>[3x]MSDIFNSPQNKASILTALMKSTTGDVEDVLIPKRFRPAKDPLDSPQAAAQFLKDNKYRILRPRAIPTMVELETDAALPRLRQMVEDGKLKDTVSVPEGTTAFYPKYYPFHKPDHDEVGTFGAPDITLLKQLTFFLLENDFPTGPETLRQVREAIATLQYGSGSYSGQLNRLLAMKGVATGRNPNKTPKTVGYTNEQLAKLLEQTLPINTPKHEDPDLRWAPSWLINYTGDLSTDKSYLPHVTIKSSAGLPYIGKTKGDTTAEALVLADSFIRDLGRAATSADPEAGVKKTITDFWYLSCGLLFPKGERYTQVDWDKKTRNIWSAPYPTHLLLSMVSTPVMNESKLNITNTQTPSLYGFSPFHGGMDRIMTIIRDSLDNDEDLVMIYADNIYILQDNTWYSIDLEKGEANCTPQHMQAMMYYLLTRGWTNEDGSPRYNPTWATFAMNVAPSMVVDSSCLLMNLQLKTYGQGSGNAFTFLNNHLMSTIVVAEWVKAGKPNPMTKEFMDLEEKTGINFKIERELKNLRETIVEAVETAPQDGYLADGSDLPPIRPGKAVELDLLGWSAIYSRQMEMFVPVLENERLIASAAYPKGLENKALARKPGAEIAYQIVRYEAIRLVGGWNNPLLETAAKHMSLDKRKRLEVKGIDVTGFLDDWNNMSEFGGDLEGITLSEPLTNQTLVDINTPLDSFDPKARPQTPRSPKKTLDE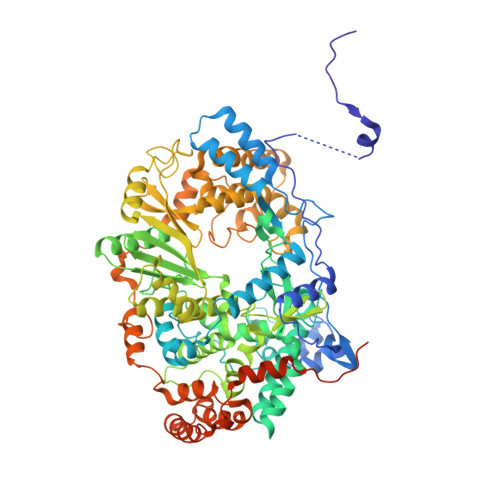VTTAITSGTYKDPKSAVWRLLDQRTKLRVSTLRDQALALKPASSSVDNWAEATEELAQQQQLLMKANNLLKSSLTETREALETIQSDKIIAGKSNPEKNPGTAANPVVGYGEFSEKIPLTPTQKKNAKRREKQRRNQVEHHHHHH;> MSDIFNSPQNKASILTALMKSTTGDVEDVLIPKRFRPAKDPLDSPQAAAQFLKDNKYRILRPRAIPTMVELETDAALPRLRQMVEDGKLKDTVSVPEGTTAFYPKYYPFHKPDHDEVGTFGAPDITLLKQLTFFLLENDFPTGPETLRQVREAIATLQYGSGSYSGQLNRLLAMKGVATGRNPNKTPKTVGYTNEQLAKLLEQTLPINTPKHEDPDLRWAPSWLINYTGDLSTDKSYLPHVTIKSSAGLPYIGKTKGDTTAEALVLADSFIRDLGRAATSADPEAGVKKTITDFWYLSCGLLFPKGERYTQVDWDKKTRNIWSAPYPTHLLLSMVSTPVMNESKLNITNTQTPSLYGFSPFHGGMDRIMTIIRDSLDNDEDLVMIYADNIYILQDNTWYSIDLEKGEANCTPQHMQAMMYYLLTRGWTNEDGSPRYNPTWATFAMNVAPSMVVDSSCLLMNLQLKTYGQGSGNAFTFLNNHLMSTIVVAEWVKAGKPNPMTKEFMDLEEKTGINFKIERELKNLRETIVEAVETAPQDGYLADGSDLPPIRPGKAVELDLLGWSAIYSRQMEMFVPVLENERLIASAAYPKGLENKALARKPGAEIAYQIVRYEAIRLVGGWNNPLLETAAKHMSLDKRKRLEVKGIDVTGFLDDWNNMSEFGGDLEGITLSEPLTNQTLVDINTPLXXXXXXXXXXXXXXXXXXXXXXXXXXXXXXXXXXXXXXXXXXXXXXXXXXXXXXXXXXXXXXXXXXXXXXXXXXXXXXXXXXX> ALPQTVRIGTDTTYAPFSSKDAKGEFIGFDIDLGNEMCKRMQVKCTWVASDFDALIPSLKAKKIDAIISSLSITDKAQQEIAFSDKLYAADSRLIAAKGSPIQPTLESLKGKHVGVLQGSTQEAYANDNWRTKGVDVVAYANQDLIYSDLTAGRLDAALQDEVAASEGFLKQPAGKEYAFAGP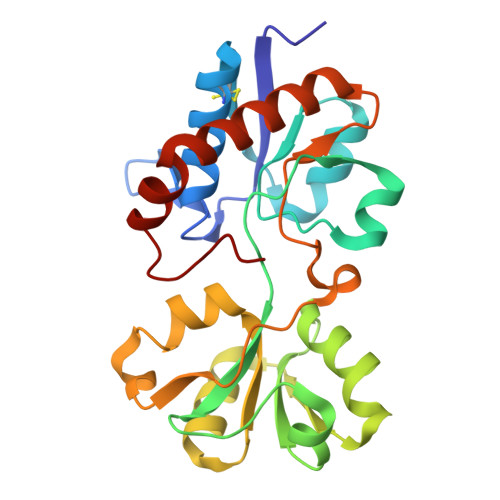SVKDKKYFGDGTGVGLRKDDTELKAAFDKALTELRQDGTYDKMAKKYFDFNVYGD>GPHAKPPYSYISLITMAIQQSPNKMLTLSEIYQ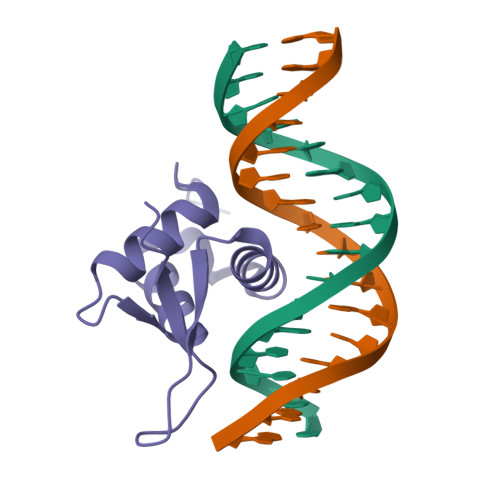WIMDLFPFYRQNQQRWQNSIRHSLSFNDCFLKVPRSPDKPGKGSFWTLHPDSGNMFENGCYLRRQKRFKCE[4x]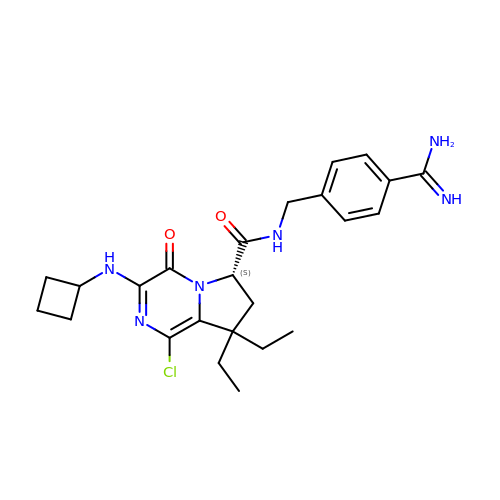(6S)-N-(4-carbamimidoylbenzyl)-1-chloro-3-(cyclobutylamino)-8,8-diethyl-4-oxo-4,6,7,8-tetrahydropyrrolo[1,2-a]pyrazine-6-carboxamide | C24 H31 Cl N6 O2 | PSBXYQNRXKCBMB-KRWDZBQOSA-N N-oxidanyl-2-[(4-phenylphenyl)sulfonylamino]ethanamide 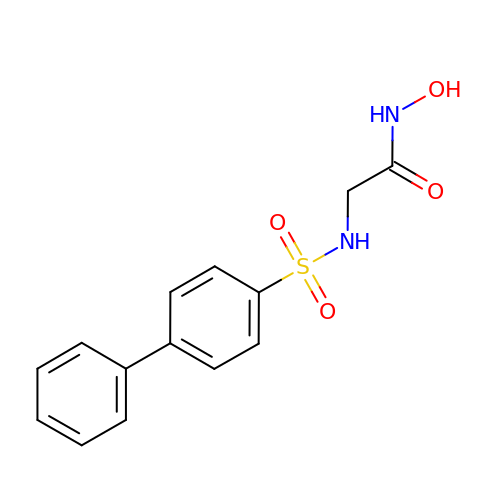| C14 H14 N2 O4 S | NKGRTRASISLCCZ-UHFFFAOYSA-N4-BENZYLBENZAMIDE 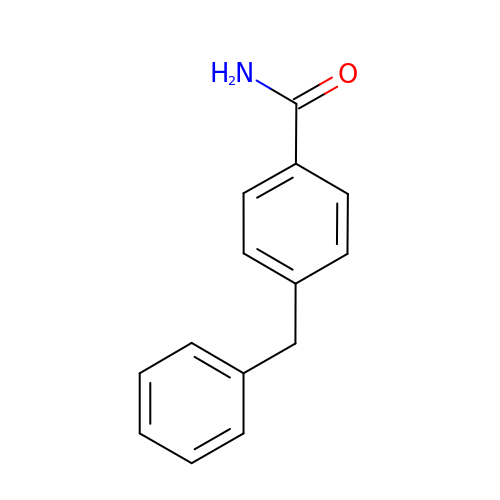| C14 H13 N O | BGTIIRYHWGADFD-UHFFFAOYSA-N>[2x]GSHMGSASEQRVTLTNADKVLYPATGTTKSDIFDYYAGVAEVMLGHIAGRPATRKRWPNGVDQPAFFEKQLALSAPPWLSRATVAHRSGTTTYPIIDSATGLAWIAQQAALEVHVPQWR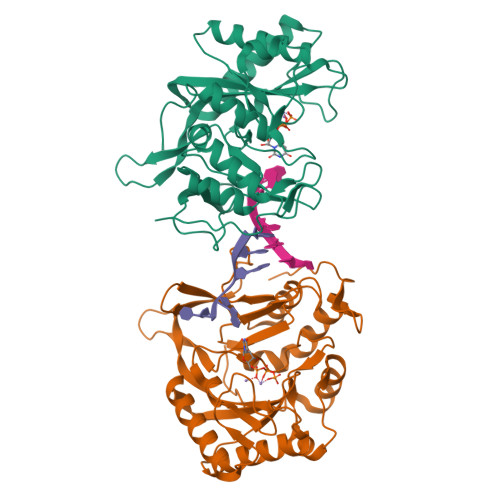FVAEPGSGELNPGPATRLVFDLDPGEGVMMAQLAEVARAVRDLLADIGLVTFPVTSGSKGLHLYTPLDEPVSSRGATVLAKRVAQRLEQAMPALVTSTMTKSLRAGKVFVDWSQNSGSKTTIAPYSLRGRTHPTVAAPRTWAELDDPALRQLSYDEVLTRIARDGDLLERLDADAPVADRLTRY>GPLGSPEFISLTSIPSLREQQHPLIRQLADCIEEVWHQHLDLSPYHLPAELGYVEGRLEGEKLTIENRCYQTPQFRKMHLELAKVGNMLDILHCVMFPRPEYDLPMFGCDLVGGRGQISAAIADLSPVHLDRTLPESYNSALTSLNTLNFSQPRELPEWGNIFSDFCIFVRPSSPEEEA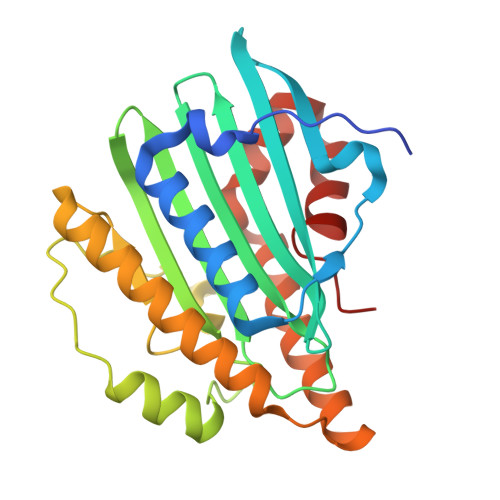MFLGRVREFLQVHCQGAIAASPVSAEQKQQILAGQHNYCSKQQQNDKTRRVLEKAFGVDWAENYMTTVLFDLPE[12x]> MDAYSTRPLTLSHGSLEHVLLVPTASFFIASQLQEQFNKILPEPTEGFAADDEPTTPAELVGKFLGYVSSLVEPSKVGQFDQVLNLCLTEFENCYLEGNDIHALAAKLLQENDTTLVKTKELIKNYITARIMAKRPFDKKSNSALFRAVGEGNAQLVAIFGGQGNTDDYFEELRDLYQTYHVLVGDLIKFSAETLSELIRTTLDAEKVFTQGLNILEWLENPSNTPDKDYLLSIPISCPLIGVIQLAHYVVTAKLLGFTPGELRSYLKGATGHSQGLVTAVAIAETDSWESFFVSVRKAITVLFFIGVRCYEAYPNTSLPPSILEDSLENNEGVPSPMLSISNLTQEQVQDYVNKTNSHLPAGKQVEISLVNGAKNLVVSGPPQSLYGLNLTLRKAKAPSGLDQSRIPFSERKLKFSNRFLPVASPFHSHLLVPASDLINKDLVKNNVSFNAKDIQIPVYDTFDGSDLRVLSGSISERIVDCIIRLPVKWETTTQFKATHILDFGPGGASGLGVLTHRNKDGTGVRVIVAGTLDINPDDDYGFKQEIFDVTSNGLKKNPNWLEEYHPKLIKNKSGKIFVETKFSKLIGRPPLLVPGMTPCTVSPDFVAATTNAGYTIELAGGGYFSAAGMTAAIDSVVSQIEKGSTFGINLIYVNPFMLQWGIPLIKELRSKGYPIQFLTIGAGVPSLEVASEYIETLGLKYLGLKPGSIDAISQVINIAKAHPNFPIALQWTGGRGGGHHSFEDAHTPMLQMYSKIRRHPNIMLIFGSGFGSADDTYPYLTGEWSTKFDYPPMPFDGFLFGSRVMIAKEVKTSPDAKKCIAACTGVPDDKWEQTYKKPTGGIVTVRSEMGEPIHKIATRGVMLWKEFDETIFNLPKNKLVPTLEAKRDYIISRLNADFQKPWFATVNGQARDLATMTYEEVAKRLVELMFIRSTNSWFDVTWRTFTGDFLRRVEERFTKSKTLSLIQSYSLLDKPDEAIEKVFNAYPAAREQFLNAQDIDHFLSMCQNPMQKPVPFVPVLDRRFEIFFKKDSLWQSEHLEAVVDQDVQRTCILHGPVAAQFTKVIDEPIKSIMDGIHDGHIKKLLHQYYGDDESKIPAVEYFGGESPVDVQSQVDSSSVSEDSAVFKATSSTDEESWFKALAGSEINWRHASFLCSFITQDKMFVSNPIRKVFKPSQGMVVEISNGNTSSKTVVTLSEPVQGELKPTVILKLLKENIIQMEMIENRTMDGKPVSLPLLYNFNPDNGFAPISEVMEDRNQRIKEMYWKLWIDEPFNLDFDPRDVIKGKDF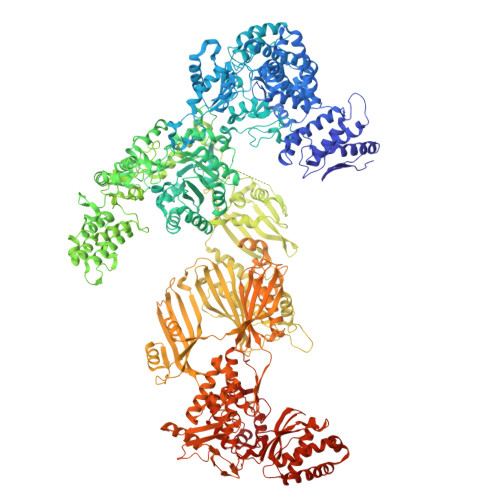EITAKEVYDFTHAVGNNCEDFVSRPDRTMLAPMDFAIVVGWRAIIKAIFPNTVDGDLLKLVHLSNGYKMIPGAKPLQVGDVVSTTAVIESVVNQPTGKIVDVVGTLSRNGKPVMEVTSSFFYRGNYTDFENTFQKTVEPVYQMHIKTSKDIAVLRSKEWFQLDDEDFDLLNKTLTFETETEVTFKNANIFSSVKCFGPIKVELPTKETVEIGIVDYEAGASHGNPVVDFLKRNGSTLEQKVNLENPIPIAVLDSYTPSTNEPYARVSGDLNPIHVSRHFASYANLPGTITHGMFSSASVRALIENWAADSVSSRVRGYTCQFVDMVLPNTALKTSIQHVGMINGRKLIKFETRNEDDVVVLTGEAEIEQPVTTFVFTGQGSQEQGMGMDLYKTSKAAQDVWNRADNHFKDTYGFSILDIVINNPVNLTIHFGGEKGKRIRENYSAMIFETIVDGKLKTEKIFKEINEHSTSYTFRSEKGLLSATQFTQPALTLMEKAAFEDLKSKGLIPADATFAGHSLGEYAALASLADVMSIESLVEVVFYRGMTMQVAVPRDELGRSNYGMIAINPGRVAASFSQEALQYVVERVGKRTGWLVEIVNYNVENQQYVAAGDLRALDTVTNVLNFIKLQKIDIIELQKSLSLEEVEGHLFEIIDEASKKSAVKPRPLKLERGFACIPLVGISVPFHSTYLMNGVKPFKSFLKKNIIKENVKVARLAGKYIPNLTAKPFQVTKEYFQDVYDLTGSEPIKEIIDNWEKYEQS>[4x]GSVWCRHCGATSAGLRCEWQNNYTQCAPCASLSSCPVCYRNYREEDLILQCRQCDRWMHAVCQNLNTEEEVENVADIGFDCSMCRPYMPASN;>SGRGKGGKGLGKGGAKRHRK[2x]

MLL3 (also called KMT2C) and MLL4 (alias KMT2D and ALR) are two closely related members of the SET1/MLL family of histone H3K4 methyltransferases, and often act as tumor suppressors. In this study, we set out to clarify the histone binding nature of the PHD6 domain in MLL3/4, and find that an extended PHD domain including the PHD6 domain and the preceding zinc finger (ePHD6) in MLL3/4 specifically recognizes an H4H18-containing fragment of histone H4. Thus, our study identifies a binding mode of the extended PHD domain of MLL3/4 for the histone H4 N-terminal fragment and provides insights into a trans-histone regulatory mechanism of MLL3/4-mediated H3K4 methylation.

The crystal structure of the MLL3 ePHD6 domain revealed that it contains a canonical PHD domain preceded by a zinc knuckle composed of two antiparallel β strands and an α helix. The MLL3 ePHD6 domain formed a dimer through two N-terminal cysteine residues, which coordinated a zinc ion (Zn0) with two cysteine residues from each protomer of the dimer. In addition, a domain swapping between these two ePHD6 molecules also contributed to the dimer formation, in which a zinc ion (Zn1) was chelated by three cysteine residues from one molecule and one histidine residue from the other molecule. The dimer involved only the preceding zinc fingers, but not the PHD domain itself. In the complex structure, the histone H4 peptide bound to one molecule of the two ePHD6 molecules and was induced to form a β strand antiparalleling with β3 of ePHD6. Of note, the β3 of ePHD6 was also induced to become longer than that in the apo molecule. The residues 14GAKRHR19 of the histone H4 peptide could be traced reliably. The H4G14, H4K16, and H4H18 residues formed main chain hydrogen bonds with the main chains of Q1102, I1100, E1097, and D1098 of MLL3, respectively, allowing the β-sheet formation between the H4 peptide and ePHD6 of MLL3. The side chain of H4A15 was accommodated in a shallow hydrophobic pocket, formed by L1101, V1123, and A1127 of MLL3, while its main chain was restricted by W1109 of MLL3. The aliphatic chain of H4K16 stacked with the aromatic ring structure of W1109 and interacted with the hydrophobic side chain of I1100.>[2x]MGSDKIHHHHHHMRKAWVKTLALDRVSNTPVVILGIEGTNRVLPIWIGACEGHALALAMEKMEFP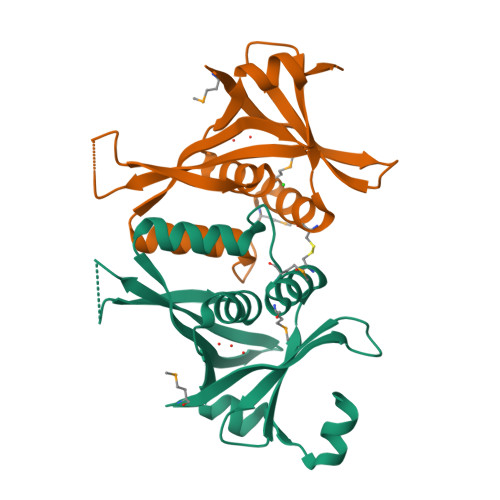RPLTHDLLLSVLESLEARVDKVIIHSLKDNTFYATLVIRDLTYTDEEDEEAALIDIDSRPSDAIILAVKTGAPIFVSDNLVEKHSIELEVNERDLINSR>GMTTATTSPVHAYQGVSDTEFSEWEQVAARVAGELSATALTRDRANQNPIAEIELLRRYGLLSFATAREFGGAGGSLVQALQLGRIIAAADGSIGQLLVYHYSNGVWTYILGSPTQREYISRGVGGHGWFQGSVSNPRDPGITVTRTEEGYRVNGKRTFATGVAVADLITVLLYEAEPINAIIPSERDGLRFNDDWDNLGQRLTASGSVEFDNVLLRHDEVLTGLDEYSGLDGSRERRDGLRALFSQLIFVHLYLGIAEGALAAGVAYIR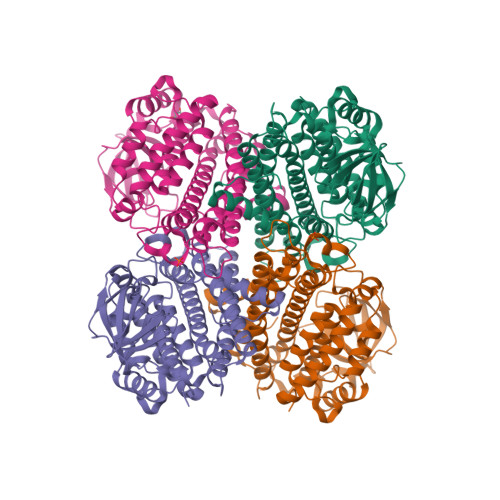DKGRPWPEAHSTDVTEDPYHQQLLGRLSAGIAAGVALADSATKEFEQALAFGEAPTEAQWGALAIRVDQAKSVATEISLDVTHNIYQATGARSTANSVGLDIYWRNARTHTTHDPLPYRQREIGRHLLTDQWPSPRSLNGLGRLAETTQGKKP[16x]>MAGAAAAVAAGAAAGAAAAAVSVAAPGRASAPPPPPPVYCVCRQPYDVNRFMIECDICKDWFHGSCVGVEEHHAVDIDLYHCPNCAVLHGSSLMKKRRNWHRHDYTEIDDGSKPVQAGTRTFIKELRSRVFPSADEIIIKMHGSQLTQRYLEKHGFDVPIMVPKLDDLGLRLPSPTFSVMDVERYVGGDKVIDVIDVARQADSKMTLHNYVKYFMNPNRPKVLNVISLEFSDTKMSELVEVPDIAKKLSWVENYWPDDSVFPKPFV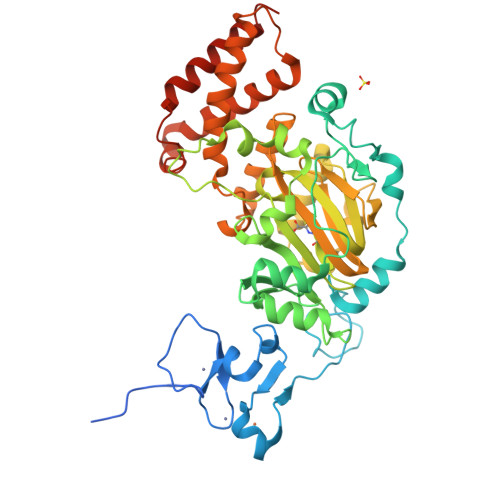QKYCLMGVQDSYTDFHIDFGGTSVWYHVLWGEKIFYLIKPTDENLARYESWSSSVTQSEVFFGDKVDKCYKCVVKQGHTLFVPTGWIHAVLTSQDCMAFGGNFLHNLNIGMQLRCYEMEKRLKTPDLFKFPFFEAICWFVAKNLLETLKELREDGFQPQTYLVQGVKALHTALKLWMKKELVSEHAFEIPDNVRPGHLIKELSKVIRAIEEENGKPVKSQGI[2x]> KFIV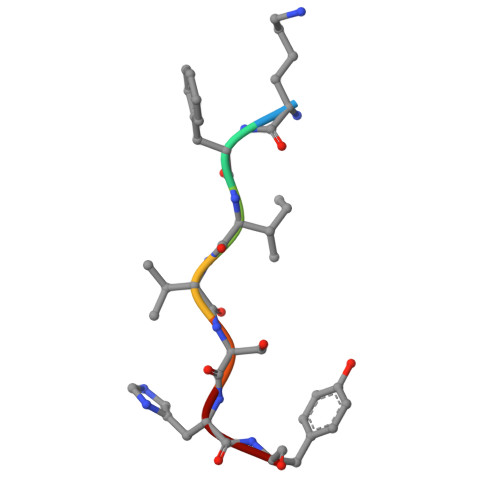SHY>[8x]MASATFTGVIPPVMTPLHADGSVDVESLRKLVDHLINGGVDGLFALGSSGEAAFLTRAQ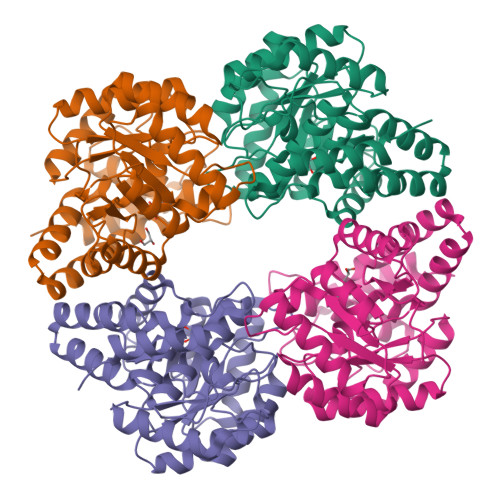RKLALTTIIEHTAGRVPVTAGVIETTTARVIELVEDALEAGAEGLVATAPFYTRTHDVEIEEHFRKIHAAAPELPLFAYNIPVSVHSNLNPVMLLTLAKDGVLAGTKDSSGNDGAIRSLIEARDDAGLTEQFKILTGSETTVDFAYLAGADGVVPGLGNVDPAAYAALAKLCLDGKWAEAAALQKRINHLFHIVFVGDTSHMSGSSAGLGGFKTALAHLGIIESNAMAVPHQSLSDEETARIHAIVDEFLYTA>SMVSPREKQQTNSKGSSNFCVKNIKQAEFGRREIEIAEQDMSALISLRKRAQGEKPLAGAKIVGCTHITAQTAVLIETLCALGAQCRWSACNIYSTQNEVAAALAEAGVAVFAWKGESEDDFWWCIDRCVNMDGWQANMILDDGGDLTHWVYKKYPNVFKKIRGIVEESVTGVHRLYQLSKAGKLCVPAMNVNDSVTKQKFDNLYCCRESILDGLKRTTDVMFGGKQVVVCGYGEVGKGCCAALKALGAIVYITEIDP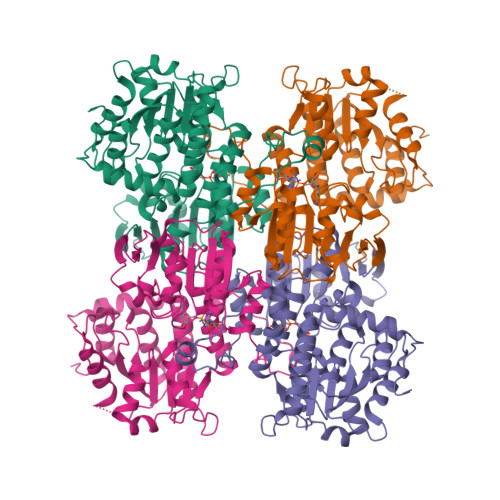ICALQACMDGFRVVKLNEVIRQVDVVITCTGNKNVVTREHLDRMKNSCIVCNMGHSNTEIDVTSLRTPELTWERVRSQVDHVIWPDGKRVVLLAEGRLLNLSCSTVPTFVLSITATTQALALIELYNAPEGRYKQDVYLLPKKMDEYVASLHLPSFDAHLTELADDQAKYLGLNKNGPFKPNYYRY[2x]The initial step involved in oxidative hydroxylation of monoaromatic and polyaromatic compounds by the microorganism Sphingobium yanoikuyae strain B1 (B1), previously known as Sphingomonas yanoikuyae strain B1 and Beijerinckia sp. strain B1, is performed by a set of multiple terminal Rieske non-heme iron oxygenases. These enzymes share a single electron donor system consisting of a reductase and a ferredoxin (BPDO-FB1). One of the terminal Rieske oxygenases, biphenyl 2,3-dioxygenase (BPDO-OB1), is responsible for B1's ability to dihydroxylate large aromatic compounds, such as chrysene and benzo[a]pyrene. Rieske oxygenase systems have multiple components whose function is to transfer electrons from NAD(P)H to active molecular oxygen and ultimately oxidize aromatic hydrocarbon substrates.

Previous structural investigations of ROs have demonstrated that substrate bound in the active site is oriented such that the carbon(s) oxidized in the dihydroxylation reaction is (are) closest to the mononuclear iron. This trend is also seen in the structure of BPDO-OB1 bound to biphenyl. The 2 and 3 carbons of biphenyl are positioned closest to the iron, with a water/hydroxide molecule bound to the iron positioned between the substrate and the iron. Crystals were grown and biphenyl was added in the presence of atmospheric oxygen. The enzyme was oxidized and no electron source was added; therefore, catalysis did not occur. We are unable to determine whether the iron is coordinated to a water molecule (hydroxide ion) or an oxygen molecule at this resolution. No significant changes in the active site main chain were observed near the mononuclear iron compared to the native structure. The loop covering the active site entrance of BPDO-OB1 shifts upon binding of biphenyl. The loop main-chain was pushed slightly away (~0.2–0.3 Å) from the substrate in the complex structure, while the main-chain proximal to the mononuclear iron remained static. Comparing the ligand bound structures, biphenyl carbons 2 and 3 are closer to the mononuclear iron in BPDO-ORHA1, 4.3 and 4.6 Å respectively, as compared to BPDO-OB1 which has an average distance of approximately 5.0 Å for both the 2 and 3 carbons in the three subunits.

>MSSDATLVDTVNASQSRQVFWDEDVYALEIERIFSRAWLMLGHESLVPKPGDFITTYMAEDKVILSHQSDGTFRAFINSCSHRGNQICHADSGNAKAFVCNYHGWVFGQDGSLVDVPLESRCYHNSLDKQKLAAKSVRVETYKGFIFGCHDPEAPSLEDYLGEFRYYLDTIWEGAGGGMELLGPPMKSLLQCNWKVPAENFIGDGYHVGWTHAAALSQIGGELAGLAGNRADIPFDDLGLQFTTRHGHGFGVIDNAAAGLHIKREGWTKFLEDTRGEVRRKFGPERERLYLGHWNCSIFPNCSFLYGTNTFKIWHPRGPHEIEVWTYTIVPRDADPATKSMIQREAIRTFGTAGTLESDDGENMSSATYINRGVITRNGRMNSTMGVGYEGPHPVYPGIVGISFIGETSYRGFYRFWKEMIDAPDWASVKANDDTWDSVFPNRNFWNEKLNAAE[3x];>[3x]MSSEQIPVTPDVHYDIEAHYRAEVRMFQTGQYREWLQGMVAEDIHYWMPIYEQRLTRDRRPDPTPDDAAIYNDDFGELKQRVERLYSGQVWMEDPPSKIRYFVSNVEAFEAGNGELDVLSNILVYRNRRQTEVTVHTLGREDKLRRDGNGFKVFRRKLILDARVTQDKNLYFFC>EPAAAPNGISLPAGYKDWKMIGVSSRIEQNNLRAILGNDIAVKAAREGRTHPWPDGAILVKLSWKKSTHELFPSAEVPGDFTQADFMVKDAAKYASTGGWGYARWLGMEQKPYGANADFAQECMGCHSGAKAADYVFTHPAKLP[2x]

Cytochromes P460 oxidise hydroxylamine within the nitrogen cycle and contain as their active site an unusual catalytic c-type haem where the porphyrin is crosslinked to the protein via a lysine residue in addition to the canonical cross links from cysteine residues. Cytochromes P460 consist of a homodimer with one haem P460 per monomer. The oxidation of hydroxylamine is a key part of the process of nitrification, whereby fixed nitrogen is converted to biologically available forms such as nitrate, in a range of bacteria. Here we describe the evidence for a novel double crosslink between lysine and haem in the cytochrome P460 from Methylococcus capsulatus (Bath).

To ascertain whether degradation of crystals over time was responsible for the variability in observed crosslinking, we collected diffraction data from crystals in situ 2 d after setting the crystallisation plate, and again 7 weeks later using other crystals from the same plate. Pleasingly, the fresh crystals yielded a structure with a clearly resolved conformation of Lys78. Since there are now four carbons bonded to C2A, they must all do so through single bonds to satisfy its valence. This means the C2A–C3A bond has been changed from double to single. The geometry around C3A remained clearly planar in the structure, so we assign it an exocyclic double bond, as evidenced by a shorter bond length to the terminal carbon on this tetrapyrrole ring D compared to all others (1.46 Å vs. 1.52 Å when using restraints without this double-bond; 1.33 Å when using double-bond restraints). We therefore tentatively built a double bond between the CD and CE carbons of Lys78 in the RT fresh and RT aged models. The RT fresh structure is very similar to the damage-free SFX structure (RMSD 0.14 Å across 286 residues).>[2x]MFQQLSARLQEAIGRLRGRGRITEEDLKATLREIRRALMDADVNLEVARDFVERVREEALGKQVLESLTPAEVILATVYEALKEALGGEARLPVLKDRNLWFLVGLQGSGKTTTAAKLALY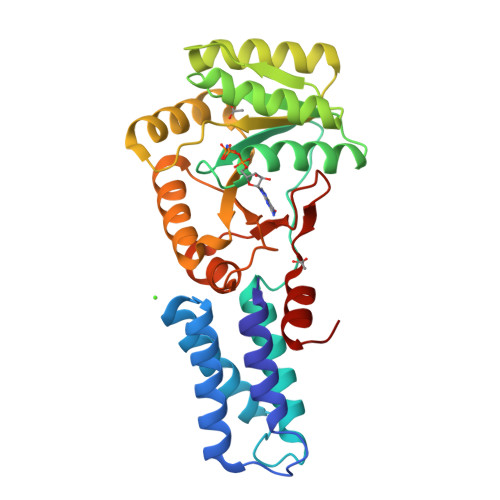YKGKGRRPLLVAADTQRPAAREQLRLLGEKVGVPVLEVMDGESPESIRRRVEEKARLEARDLILVDTAGRLQIDEPLMGELARLKEVLGPDEVLLVLDAMTGQEALSVARAFDEKVGVTGLVLTKLDGDARGGAALSARHVTGKPIYFAGVSEKPEGLEPFYPERLAGRILGMGD>[4x]SNALLSQRSAWFPRPVAAPAAEPPDPAAAPLRLVCFPYA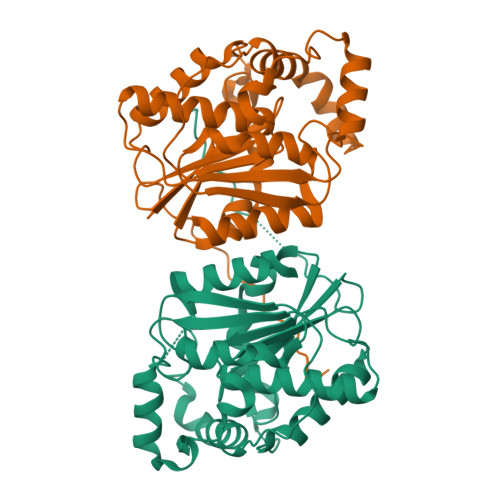GGTVSAFRGWQERLGDEVAVVPVQLPGRGLRLRERPYDTMEPLAEAVADALEEHRLTHDYALFGHSMGALLAYEVACVLRRRGAPRPRHLFVSGSRAPHLYGDRADHTLSDTALREVIRDLGGLDDADTLGAAYFDRRLPVLRADLRACERYDWHPRPPLDCPTTAFSAAADPIATPEMVEAWRPYTTGSFLRRHLPGNHFFLNGGPSRDRLLAHLGTEL>SMPKTISVRVTTMDAELEFAIQPNTTGKQLFDQVVKTIGLREVWFFGLQYQDTKGFSTWLKLNKKVTAQDVRKESPLLFKFRAKFYPEDVSEELIQDITQRLFFLQVKEGILNDDIYCPPETAVLLASYAVQSKYGDFNKEVHKSGYLAGDKLLPQRVLEQHKLNKDQWEERIQVWHEEHRGMLREDAVLEYLKIAQDLEMYGVNYFSIKNKKGSELWLGVDALGLNIYEQNDRLTPKIGFPWSEIRNISFNDKKFVIKPIDKKAPDFVFYAPRLRINKRILALCMGNHELYMRRRKPDTIEVQQMKAQARE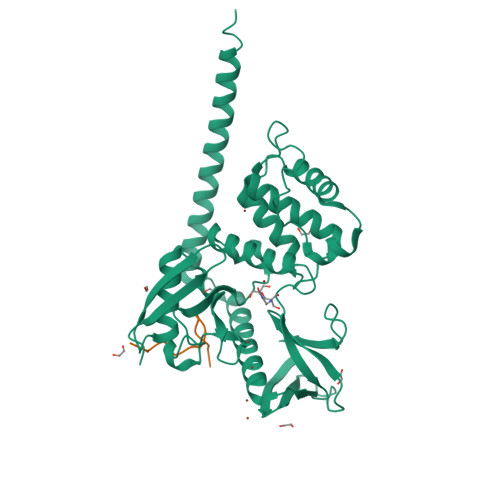EKHQKQMERAMLENEKKKREMAEKEKEKIEREKEE[2x];>EDGGSWKYPDAFELSG[2x]>[2x]GVGYKVKSTTTACCDSCVCTKSIPPQCRCNDMGETCHSACKQCICALSYPP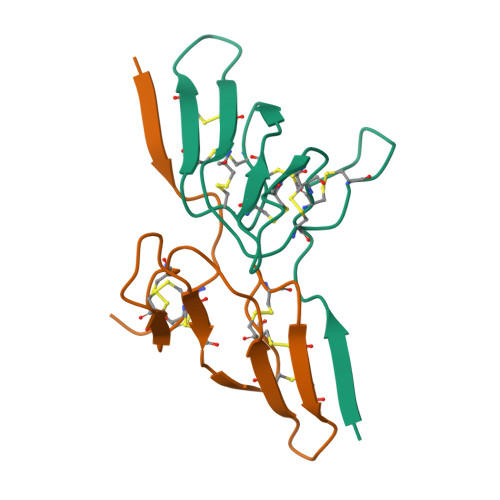ICRCMDNTGFCYDSCSKSKDQD(2~{R})-1-[4-(4-ethanoyl-3-ethyl-5-methyl-1~{H}-pyrrol-2-yl)-1,3-thiazol-2-yl]-~{N}-(4-oxidanylbutyl)piperazine-2-carboxamide | C21 H31 N5 O3 S | 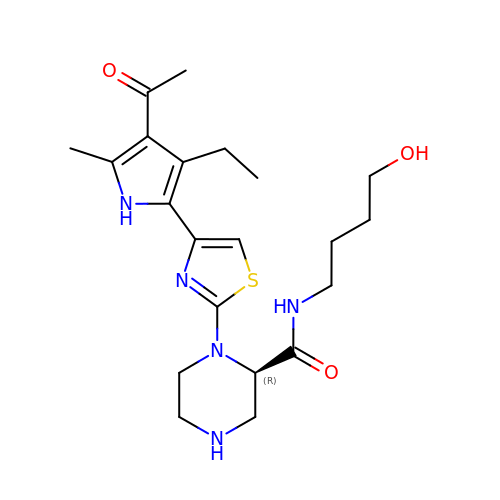BZHIMJWVFLBIRF-QGZVFWFLSA-N Repair of Iron Center proteins (RIC) form a family of di-iron proteins that are widely spread in the microbial world. RICs contain a binuclear nonheme iron site in a four-helix bundle fold, two basic features of hemerythrin-like proteins. YtfE has an L-shaped two-domain architecture: it exhibits an N-terminal ScdA_N domain connected through a highly flexible penta-peptide to the C-terminal four-helix bundle hemerythrin-like domain containing the di-iron site. Altogether the data so far gathered for YtfE such as the induction by NO stress, the interaction of YtfE with Dps and proteins of the iron-sulfur biogenesis system, the iron donor properties of YtfE, and the ability of YtfE to promote the formation of an iron-sulfur center in IscU and ferredoxin, all indicate that YtfE is a bacterial iron donor.

We also provide a new structure of the Escherichia coli YtfE in which the iron binuclear center is replaced by manganese ions and discuss its impact on the overall structure. For this purpose, wild type YtfE was incubated with Mn2+ ions during the crystallization process and X-ray diffraction data were collected. Analysis of the anomalous difference maps obtained from data collected above the Mn and Fe K-absorption edges shows that the metal site contains in both positions a mixture of iron and manganese ions: in position 2, which is closer to E159, manganese represented ca. 45% of the metal occupation, while position 1 retained almost all the iron, as only ca. 10% of manganese was present. Therefore, iron in position 2 is more easily displaced by manganese than that in position 1. This observation is consistent with the Mössbauer data showing that in YtfE one of the iron atoms is more labile. Hence it was of relevance to determine the affinity of the wild type YtfE to manganese and compare it with that of iron. This study was done by analyzing the quenching of the intrinsic fluorescence intensity of YtfE upon the addition of Mn2+ or Fe2+, and determination of the binding constants for each metal. Moreover, the binding affinity constants of the wild type and mutated protein are significantly higher for iron than for manganese (ka = 6.5 ± 0.3 × 10−6 M (Fe2+) and 0.5 ± 0.2 × 10−6 M (Mn2+)).

>[2x]MAYRDQPLGELALSIPRASALFRKYDMDYAAGGKQTLARAAARKELDVEVIEAELAKLAEQPIEKDWRSAPLAEIIDHIIVRYHDRHREQLPELILQATKVERVHADKPSVPKGLTKYLTMLHEELSSHMMKEEQILFPMIKQGMGSQAMGPISVMESEHDEAGELLEVIKHTTNNVTPPPEACTTWKAMYNGINELIDDLMDHISLENNVLFPRALAGE6-(2-{3-[2-(2-amino-6-methylpyridin-4-yl)ethyl]phenyl}ethyl)-4-methylpyridin-2-amine | C22 H26 N4 | 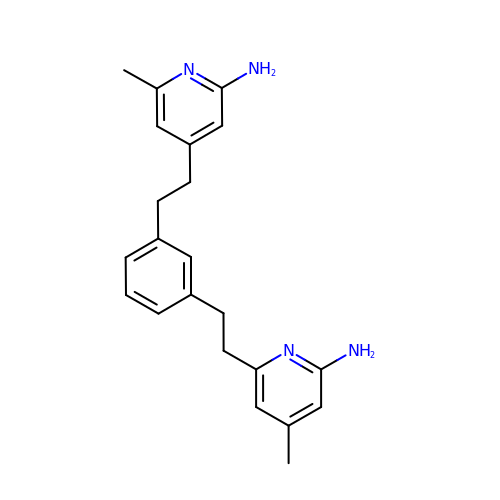JVYPSLPLMFVFFX-UHFFFAOYSA-N>[3x]MFEARLVQGSILKKVLEALKDLINEACWDISSSGVNLQSMDSSHVSLVQLTLRSEGFDTYRCDRNLAMGVNLTSMSKILKCAGNEDIITLRAEDNADTLALVFEAPNQEKVSDYEMKLMDLDVEQLGIPEQEYSCVVKMPSGEFARISRDLSHIGDAVVISCAKDGVKFSASGELGNGNIKLSQTSNVDKEEEAVTIEMNEPVQLTFALRYLNFFTKATPLSSTVTLSMSADVPLVVEYKIADMGHLKYYLAPKIEDEEGS

pmcProliferating cell nuclear antigen (PCNA) is a sliding clamp protein that acts as a molecular “hub” for chromosomal DNA replication, repair, and maintenance. PCNA consists of three identical subunits that form a closed ring that surrounds DNA. Each subunit contains one partner binding region that various factors use to interact with PCNA, allowing the trimeric ring to accommodate up to three partners simultaneously. Beyond its role in enzymatic processivity, PCNA functions as a scaffold that congregates various factors that copy, surveil, and repair DNA; thus, PCNA coordinates DNA replication with DNA repair, chromatin remodeling, cell cycle regulation, and apoptosis.

Here, we report a second PCNA substitution (C148S) that also causes PARD. We found that overall the structure of PCNA-C148S is similar to that of PCNA-WT with an RMSD value of 0.85 Å, indicating no significant global changes to the structure. Furthermore, the conformation of residues surrounding C148S does not differ significantly from PCNA-WT. Although the S228I variant has a deformed partner binding cleft, this region is not obviously altered in PCNA-C148S. It is important to note that a portion of the binding cleft exhibits weak density in our PCNA-C148S structure. Despite this issue, there is unambiguous density for Y133, a residue that dictates the conformation of the partner binding cleft. Because Y133 is in the same conformation as seen in PCNA-WT, we conclude that the partner binding cleft is unchanged in PCNA-C148S. From a structural point, the C148 residue is buried in a hydrophobic pocket near the interface between subunits and participates in a π-sulfur interaction with F144. These types of interactions have been shown to confer substantial protein stability. We found that all three PCNA variants display unfolding curves consistent with a two-state unfolding mechanism. Both PCNA-C148S and -S228I have dramatically reduced thermal stability compared with PCNA-WT (PCNA-WT Tm: 52.0 ± 0.03 °C, PCNA-C148S Tm: 42.0 ± 0.06 °C, and PCNA-S228I Tm: 44.0 ± 0.1 °C). Our combined structural and affinity binding studies indicate that, in contrast to PCNA-S228I, PCNA-C148S does not exhibit the defect in partner binding that was thought to drive PARD.CTP synthase (CTPS) catalyzes the final, rate-limiting step of de novo CTP biosynthesis (Lieberman, 1956). Each CTPS monomer consists of a glutaminase domain and an amido-ligase domain connected by an alpha helical linker. Glutamine hydrolysis in the glutaminase domain produces ammonia which is transferred through a channel into the amido-ligase domain, where it is ligated to UTP to form CTP in an ATP-dependent process. Budding yeast have two CTPS isoforms, Ura7 and Ura8, which share 78 % identical residues.

We determined structures of CTPS filament bundles formed at pH 6.0 to better understand the mechanisms of lateral assembly. Reference-free two-dimensional averages of bundle segments from cryo-EM images of Ura7 and Ura8 were strikingly regular, suggesting ordered assembly contacts. This high degree of order allowed us to determine three-dimensional structures of both homologs in the presence of substrates or product using a single particle reconstruction approach by focused refinement of interacting pairs of filaments. As we found for the single filament structures, Ura8 reconstructions went to higher resolution (3.3 Å for substrates and 3.7 Å for product) than Ura7 (6.6 Å substrate and 7.0 Å product). The individual filaments that pack laterally in the bundles closely resemble the corresponding single filament structures. Ura7 formed very similar bundles in both ligand conditions, with adjacent filaments staggered relative to each other with a half-tetramer offset. Although at lower resolution, the Ura7 structures appear to make the same lateral contacts as substrate-bound Ura8. Yeast CTPS has a 7-residue insert (residues 273–279) in the linker region that mediates the bulk of the lateral interaction in both bundle types. Ura7 bundles in either ligand state are very similar, and at our resolution appear to maintain the same lateral contacts but with a slightly different helical twist. Regardless of nucleotide pools, bundles could therefore remain assembled to fulfill their role in the starvation response.

>[28x]MKYVVVSGGVISGIGKGVLASSTGMLMKTLGLKVTSIKIDPYMNIDAGTMSPLEHGECFVLDDGGETDLDLGNYERYLGVTLTKDHNITTGKIYSHVIAKERKGDYLGKTVQIVPHLTNAIQDWIERVAKIPVDDTGMEPDVCIIELGGTVGDIESAPFVEALRQFQFKVGKENFALIHVSLVPVIHGEQKTKPTQAAIKGLRSLGLVPDMIACRCSETLDKPTIDKIAMFCHVGPEQVVNVHDVNSTYHVPLLLLEQKMIDYLHARLKLDEITEEEKQRGLELLSKWKATTGNFDEETVKIALVGKYTNLKDSYLSVIKALEHSSMKCRRKLDIKWVEATDLEPEAQESNKTKFHEAWNMVSTADGILIPGGFGVRGTEGMVLAARWARENHIPFLGVCLGLQIATIEFTRSVLGRKDSHSAEFYPDIDEKNHVVVFMMRLGLRPTFFQNETEWSQIKKLYGDVSEVHERHRHRYEINPKMVDELENNGLIFVGKDDTGKRCEILELKNHPYYIATQYHPEYTSKVLDPSKPFLGLVAASAGILQDVIEGKYDLEA>EFPIIERSIRMSNPWKAFMEKYDLERAHNSGIRIDLGEDAEVGNSKYRIPAGKCPVFGKGIVIENSKVSFLTPVATGAQRLKEGGFAFPNADDHISPITIANLKERYKENADLMKLNDIALCKTHAASFVIAEDQNTNYRHPAVYDEKEKTCYMLYLSAQENMGPRYCSPDSQNKDAMFCFKPDKNEKFDNLVYLSKNVRNDWENKCPRKNLGNAKFGLWVDGNCEEIPYVNEVEARSLRECNRIVFEASASDQPRQYEEELTDYEKIQEGFRQNNRDMIKSAFLPVGAFNSDNFKSKGRGY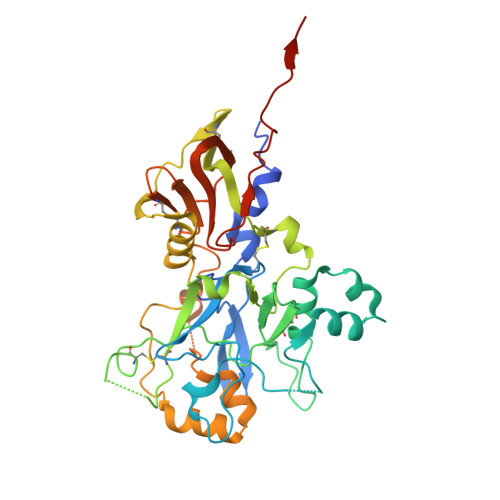NWANFDSVNNKCYIFNTKPTCLINDKNFFATTALSHPQEVDNEFPGLEQKLISEEDLNSAVDHHHHHH[2x]O-tert-butyl-N-[(3-{[(2,4,6-trimethylphenyl)carbamoyl]amino}naphthalen-2-yl)carbonyl]-L-threonine | C29 H35 N3 O5 | 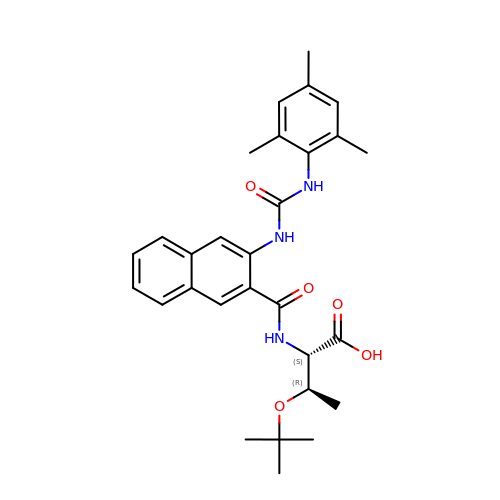SIVVDUDKHBTSKI-CLOONOSVSA-N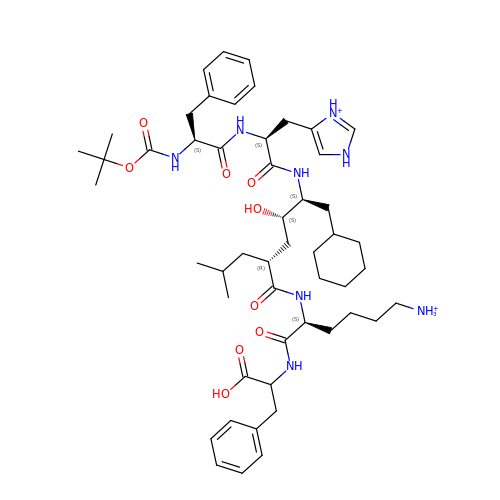6-ammonio-N-[(2R,4R,5R)-5-{[N-(tert-butoxycarbonyl)-L-phenylalanyl-3-(1H-imidazol-3-ium-4-yl)-L-alanyl]amino}-6-cyclohexyl-4-hydroxy-2-(2-methylpropyl)hexanoyl]-L-norleucylphenylalanine | C51 H78 N8 O9 | YHLJEWZZOJLRNJ-OBSKRNKISA-P> DQGIVIYNAQHENLVKSWVDGFTKDTGIKVTLRNGGDSELGNQLVQEGSASPADVFLTENSPAMVLVDNAKLFAPLDAATLAQVEPQYRPSHGRWIGIAARSTVFVYNPAKLSDAQLPKSLLDLAKPEWKGRWAASPSGADFQAIVSALLELKGEKATLAWLKAMKTNFTAYKGNSTVMKAVNAGQVDSGVIYH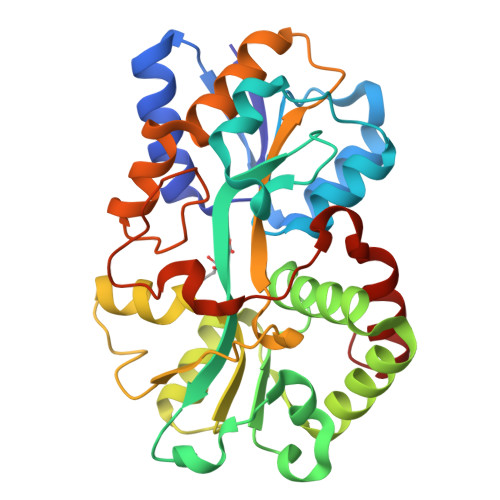YYPFVDGAKTGENSNNIKLYYFKHQDPGAFVSISGGGVLASSKHQQQAQAFIKWITGKQGQEILRTNNAFEYAVGVGAASNPKLVPLKDLDAPKVDAAQLNSKKVVELMTEAGLL[(5,7-dibromo-2-oxo-1,2-dihydroquinolin-4-yl)methyl]phosphonic acid | C10 H8 Br2 N O4 P | 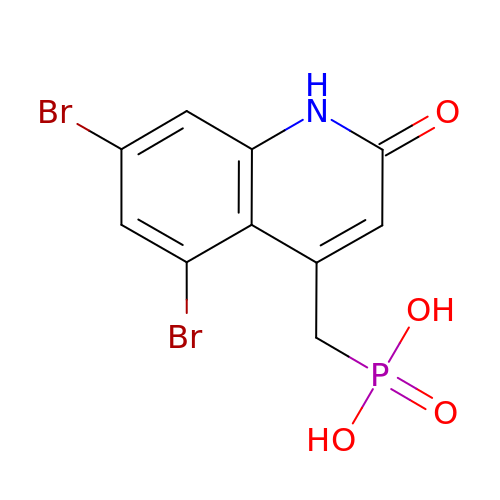YMPWKSWKTYLHON-UHFFFAOYSA-N>MHHHHHHGSMSNEQTFIAIKPDGVQRGLIGPIISRFENRGFKLVAMKLVSPPQSQLEQHYADLSDKPFFKGLVSYMLSGPICAMVWEGRDVVKTGRTILGATNPLASAPGTIRGDFAIDVGRNVCHGSDSVENAKKEI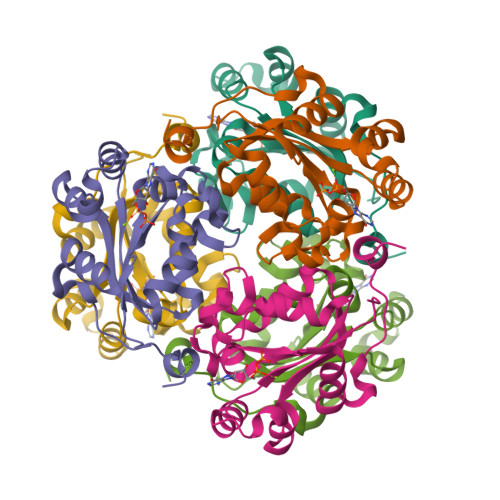ALWFKPEELISWKSATFDWVYEKA[3x]> MLHTLHRSPWLTDFAALLRLLSEGDELLLLQDGVTAAVDGNRYLESLR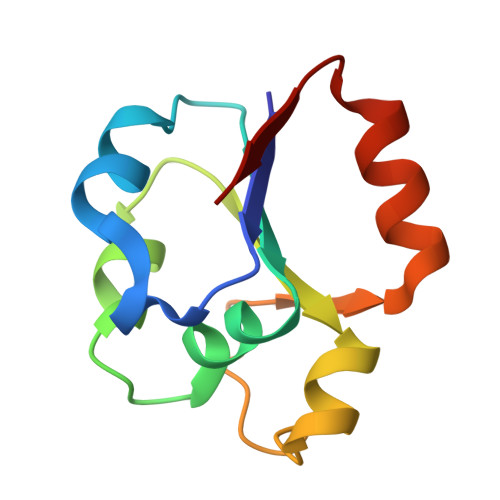NAPIKVYALNEDLIARGLTGQISNDIILIDYTDFVRLTVKHPSQMAW> IKGGLFADIASHPWQAAIFAKHRRSPGERFLCGGILISSCWILSAAHCFQERFPPHHLTVILGRTYRVVPGEEEQKFEVEKYIVHKEFDDDTYDNDIALLQLKSDSSRCAQESSVVRTVALPPADLQLPDWTECELSGYGKHEALSPEYSERLKEAHVRLYPSSRCTSQHLLQRTVTDNMLCAGDTRSGGPQANLHDACQGDAGGPLVCLNDGRMTLVGIISWGLGCGQKDVPGVYTKVTNYLDWIRDNMR;> SYVAHLASDFGVRVFQQVAQASKDRNVVFSPYGVASVLAMLQLTTGGETQQQIQAAMGFKIDDKGMAPALRHLYKELMGPWNKDEISTTDAIFVQRDLKLVQGFMPHFFRLFRSTVKQVDFSEVERARFIINDWVKTHTKGMISHLLGTGAVDQLTRLVLVNALYFNGQWKTPFPDSSTHRRLFHKSDGSTVSVPMMAQTNKFNYTEFTTPDGHYYDILELPYHGDTLSMFIAAPYEKEVPLSALTNILSAQLISHWKGNMTRLPRLLVLPKFSLETEVDLRKPLENLGMTDMFRQFQADFTSLSDQEPLHVALA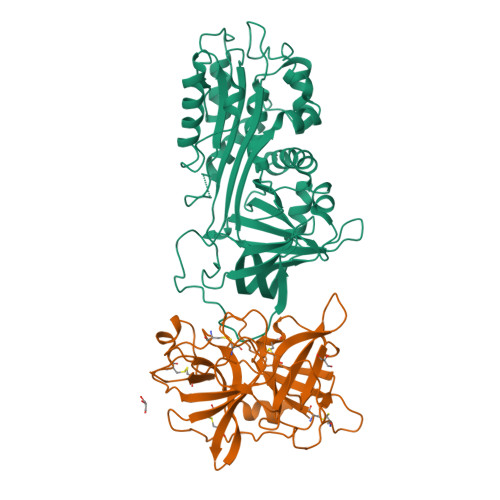LQKVKIEVNESGTVASSSTAVIVSARMAPEEIIIDRPFLFVVRHNPTGTVLFMGQVMEP>ACHPRLSLHRPALEDLLLGSEANLTCTLTGLRDASGVTFTWTPSSGKSAVQGPPERDLCGCYSVSSVLPGCAEPWNHGKTFTCTAAYPESKTPLTATLSKSGNTFRPEVHLLPPPSEELALNELVTLTCLARGFSPKDVLVRWLQGSQELPREKYLTWASRQEPSQGTTTFAVTSILRVAAEDWKKGDTFSCMVGHEALPLAFTQKTIDRLAGK[2x];>QEGDFPMPFISAKSSPVIPLDGSVKIQCQAIREAYLTQLMIIKNSTYREIGRRLKFWNETDPEFVIDHMDANKAGRYQCQYRIGHYRFRYSDTLELVVTGLYGKPFLSADRGLVLMPGENISLTCSSAHIPFDRF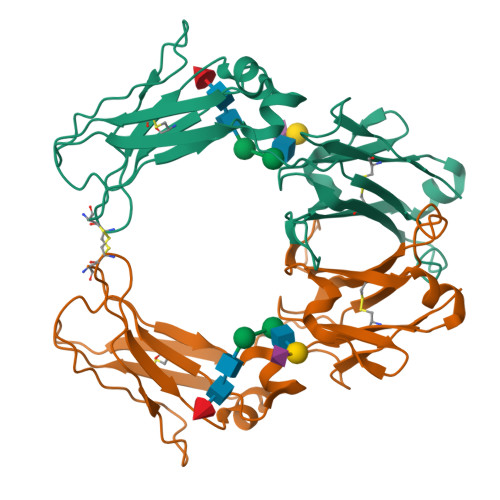SLAKEGELSLPQHQSGEHPANFSLGPVDLNVSGIYRCYGWYNRSPYLWSFPSNALELVVTAIDGRAHHHHHH[2x]>[2x]PAVESRLVGGSSICEGTVEVRQGAQWAALCDSSSAR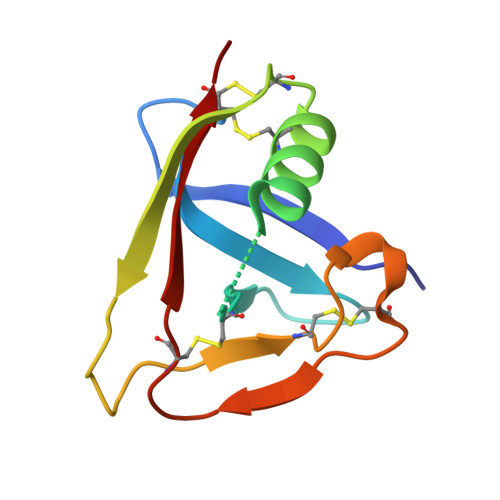SSLRWEEVCREQQCGSVNSYRVLDAGDPTSRGLFCPHQKLSQCHELWERNSYCKKVFVTCQD> MENVVSAPMPGKVLRVLVRVGDRVRVGQGLLVLEAMKMENEIPSPRDGVVKRILVKEGEY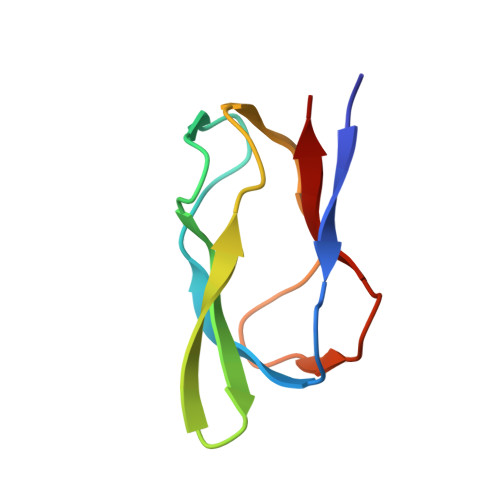VDTGQPLIELG> MSGGLLKAL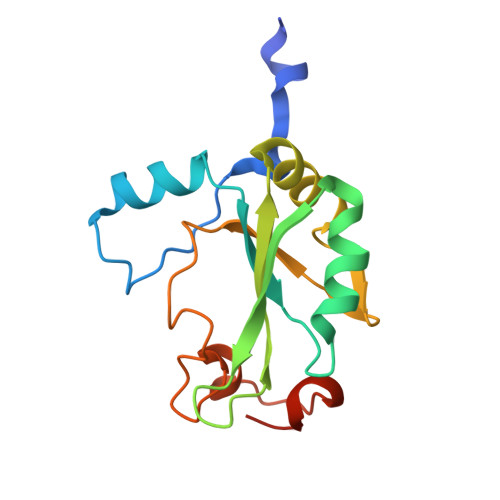RSDSYVELSQYRDQHFRGDNEEQEKLLKKSCTLYVGNLSFYTTEEQIYELFSKSGDIKKIIMGLDKMKKTACGFCFVEYYSRADAENAMRYINGTRLDDRIIRTDWDAGFKEGRQYGRGRSGGQVRDEYRQDYDAGRGGYGKLAQNQ4-({4-methoxy-6-[2-(morpholin-4-yl)ethoxy]-1,3,5-triazin-2-yl}amino)-2-(3-methylbutoxy)benzonitrile | C22 H30 N6 O4 | 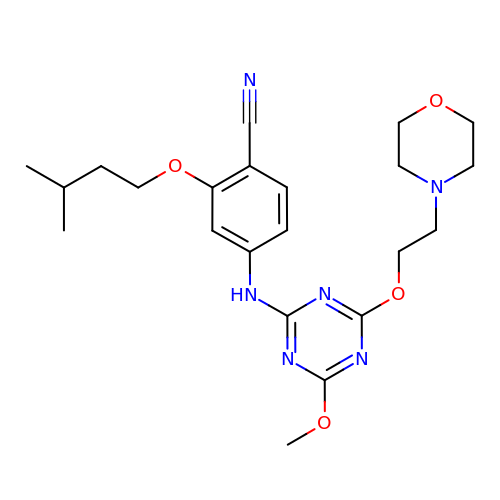VZBHPTCAQDOYJZ-UHFFFAOYSA-N> MEFSQIPASEQETLVRPKPLLLKLLKSVGAQKDTYTMKEVLFYLGQYIMTKRLYDE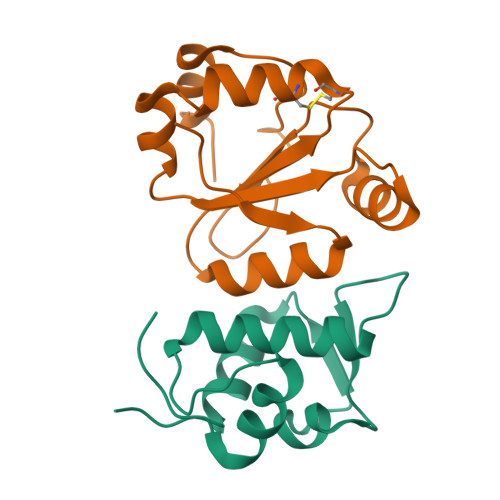KQQHIVYCSNDLLGDLFGVPSFSVKEHRKIYTMIYRNLVVVNQQESSDSGTSVSENLE;> MATHTAQTQTHLNFTQIKTAFALYWALLEAQGKPVMLDLYADWCVACKEFEKYTFSDPQVQKALADTVLLQANVTANDAQDVALLKHLNVLGLPTILFFDGQGQEHPQARVTGFMDAETFSAHLRDRQPLEHHHHHH>GGVGHWSYHGETGPQHWGDLKNEYIMCKIGKNQSPVDISRIVEAELEKIKINYSSGGSSITNNGHTIKVSYEPGSYIIVDGIRFELKQFHFHAPSEHTIKGKSYPFEAHFVHADKDGNLAVIGVIFKEGKKNPIIEKIWENLPEAGKTIKLAHKINAYDLLPKKKKYYRYSGSLTTPPCSEGVRWIVMEEEMELSKEQIEKFRKLMGGDTNRPVQ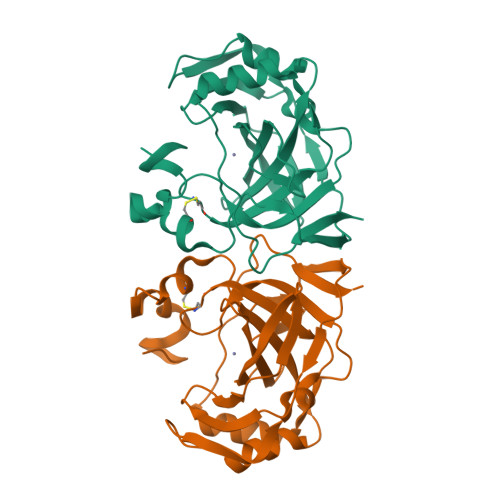PLNARMIMEMD[6x]>MAQQKKTIAVVNATGRQAASLIRVAAAVGHHVRAQVHSLKGLIAEELQAIPNVTLFQGPLLNNVPLMDTLFEGAHLAFINTTSQAGDEIAIGKDLADAAKRAGTIQHYIYSSMPDHSLYGPWPAVPMWAPKFTVENYVRQLGLPSTFVYAGIYNNNFTSLPYPLFQMELMPDGTFEWHAPFDPDIPLPWLDAEHDVGPALLQIFKDGPQKWNGHRIALTFETLSPVQVCAAFSRALNRRVTYVQVPKVEIKVNIPVGYREQLEAIEVVFGEHKAPYFPLPEFSRPAAGSPKGLGPANGKGAGAGMMQGPGGVISQRVTDEARKLWSGWRDMEEYAREVFPIEEEANGL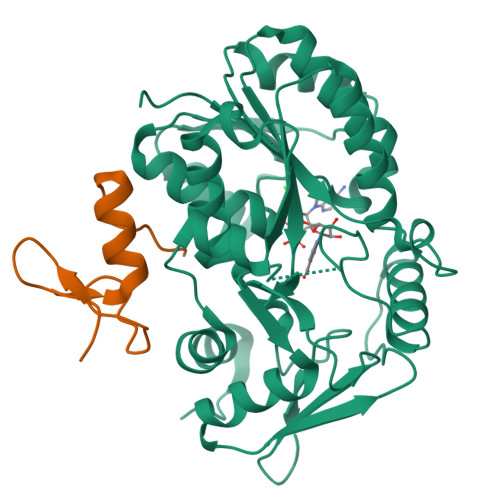DWML[8x];>[8x]PTTCTNCFTQTTPLWRRNPEGQPLCNACGLFLKLHGVVRPLSL Sterile alpha motif and HD domain containing protein 1 (SAMHD1) is a dNTP triphosphohydrolase enzyme that catalyzes the hydrolysis of dNTPs into triphosphate and 2′-deoxynucleoside. In terminally differentiated myeloid lineage cells and resting T-cells, SAMHD1 activity reduces the dNTP pool to a level that inhibits the replication of HIV-16−8 and other retroviruses as well as some DNA viruses. It comprises an N-terminal nuclear localization signal, a sterile alpha motif (SAM) domain, and an HD phosphohydrolase domain25 containing the active site. The active form of SAMHD1 is a homotetramer28 where sequences N- and C-terminal to the HD domain stabilize intersubunit protein–protein interactions and incorporate four pairs of allosteric nucleotide-binding sites, AL1 and AL2, that regulate the enzyme through combined binding of G-based (AL1) and deoxynucleoside (AL2) triphosphates. The allosteric regulation of SAMHD1 has been studied extensively.

To further investigate this preference, we cocrystallized the catalytic domain, residues 109–626, of a catalytically inactive H215A SAMHD1 mutant44 with Rp-dGTPαS and magnesium ions. The structure of this H215A-SAMHD1(109–626)-Rp-dGTPαS–Mg complex was determined by molecular replacement to 2.3 Å resolution and contains two SAMHD1 tetramers in the asymmetric unit with electron density for nucleotides and metal ions found in each of the allosteric and active sites. The H215A-SAMHD1(109–626)-Rp-dGTPαS crystal structure contains a Rp-dGTPαS substrate bound at the active site, as well as in allosteric sites AL1 and AL2. In this structure, the active site Rp-dGTPαS coordinates the His/Asp-bound Fe, two Mg ions (Mg2 and Mg3), and hydrating water molecules. Several amino acids also interact with or pack against the guanine base, 2′-deoxyribose and thio-substituted triphosphate, including Gln149, Arg164, His210, Lys312, Tyr315, Arg366, and Tyr374. Although Ala215, that replaces histidine in the H215A mutant, cannot provide the general acid required for catalysis of the substrate Rp-dGTPαS, an Fe/Mg3-bridged water, W0, that could act as a nucleophile for catalysis is positioned in line with the scissile Pα–O5′ phosphoester bond of the substrate Rp-dGTPαS. This suggests that the Rp-dGTPαS substrate conformation in the active site is representative of the precatalytic state and is consistent with our enzymological data, which demonstrates that the Rp-dNTPαS diastereomers are substrates, albeit with a small reduction in kcat relative to canonical dNTPs. In the Rp-dGTPαS structure, the Fe is coordinated by the α-phosphorothioate sulfur rather than the phosphate oxygen present in a canonical dNTP substrate. Here, it is apparent that AL1 selectivity for Rp-dGTPαS results from the α-phosphate O2A oxygen of the AL1-bound nucleotide that coordinates the AL1-AL2-bridging magnesium ion (Mg1).

>GSQIHVDTMKVINDPIHGHIELHPLLVRIIDTPQFQRLRYIKQLGGGYYVFPGASHNRFEHSLGVGYLAGCLVHALGEKQPELQISERDVLCVQIAGLCHDLGHGPFSAMFDGRFIPLARPEVKWTHEQGSVMMFEHLINSNGIKPVMEQYGLIPEEDICFIKEQIVGPLESPVEDSLWPYKGRPENKSFLYEIVSNKRNGIDVDKWDYFARDCHHLGIQNNFDYKRFIKFARVCEVDNELRICARDKEVGNLYDMFHTRNSLHRRAYQHKVGNIIDTMITDAFLKADDYIEITGAGGKKYRISTAIDDMEAYTKLTDNIFLEILYSTDPKLKDAREILKQIEYRNLFKYVGETQPTGQIKIKREDYESLPKEVASAKPKVLLDVKLKAEDFIVDVINMDYGMQEKNPIDHVSFYCKTAPNRAIRITKNQVSQLLPEKFAEQLIRVYCKKVDRKSLYAARQYFVQWCADRNFTKPQDGDVIAPLITPQKKEWNDSTSVQNPTRLREASKSRVQLFKDDPM[8x]> AVYVVGGSGGWTFNTE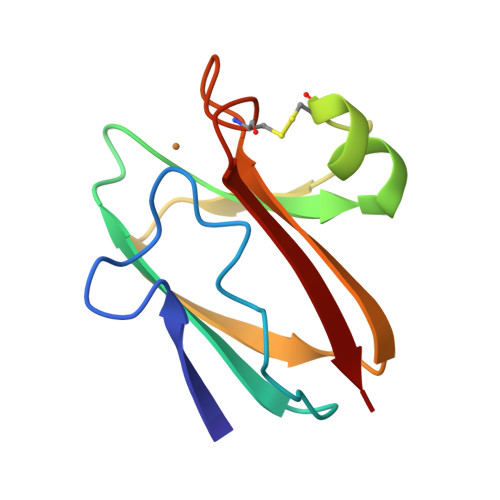SWPKGKRFRAGDILLFNYNPSMHNVVVVNQGGFSTCNTPAGAKVYTSGRDQIKLPKGQSYFICNFPGHCQSGMKIAVNAL(5Z,8Z,11Z,14Z,17R,18R)-17,18-dihydroxyicosa-5,8,11,14-tetraenoic acid | C20 H32 O4 | 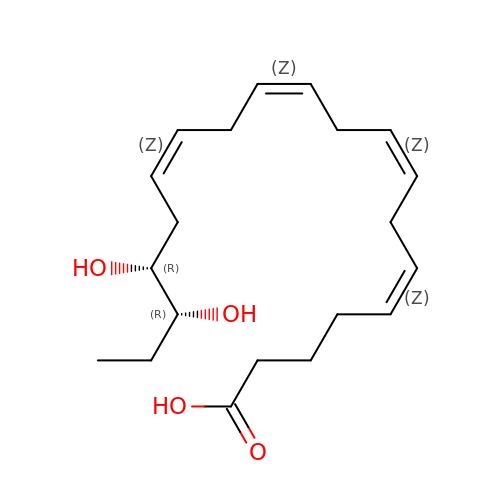XYDVGNAQQFWZEF-VXNZHGHESA-N>[12x]MAQNLKDLAGRLPAGPRGMGTALKLLLGAGAVAYGVRESVFTVEGGHRAIFFNRIGGVQQDTILAEGLHFRIPWFQYPIIYDIRARPRKISSPTGSKDLQMVNISLRVLSRPNAQELPSMYQRLGLDYEERVLPSIVNEVLKSVVAKFNASQLITQRAQVSLLIRRELTERAKDFSLILDDVAITELSFSREYTAAVEAKQVAQQ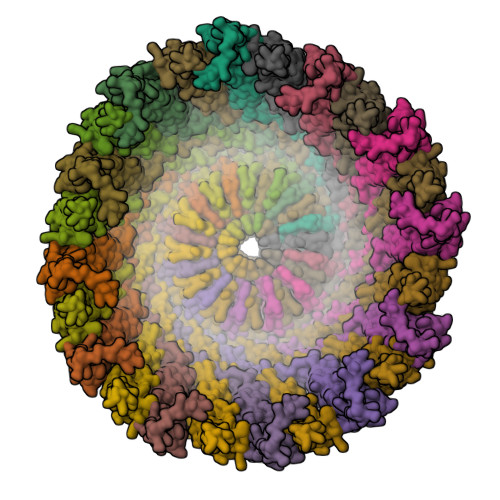EAQRAQFLVEKAKQEQRQKIVQAEGEAEAAKMLGEALSKNPGYIKLRKIRAAQNISKTIATSQNRIYLTADNLVLNLQDESFTRGSDSLIKGKK;>MAAKVFESIGKFGLALAVAGGVVNSALYNVDAGHRAVIFDRFRGVQDIVVGEGTHFLIPWVQKPIIFDCRSRPRNVPVITGSKDLQNVNITLRILFRPVASQLPRIFTSIGEDYDERVLPSITTEILKSVVARFDAGELITQRELVSRQVSDDLTERAATFGLILDDVSLTHLTFGKEFTEAVEAKQVAQQEAERARFVVEKAEQQKKAAIISAEGDSKAAELIANSLATAGDGLIELRKLEAAEDIAYQLSRSRNITYLPAGQSVLLQLPQ[12x]HEPTANE | C7 H16 | 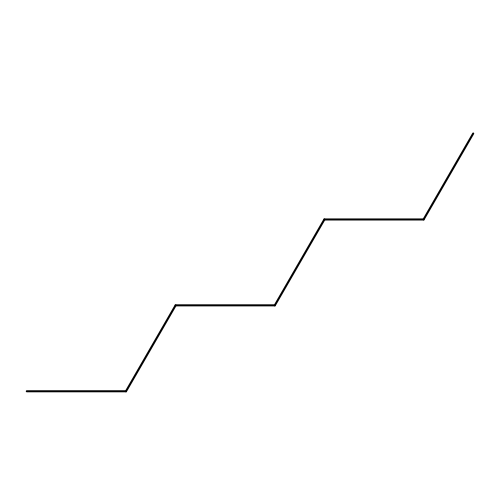IMNFDUFMRHMDMM-UHFFFAOYSA-N>GSQGHDTVQPNFQQDKFLGRWY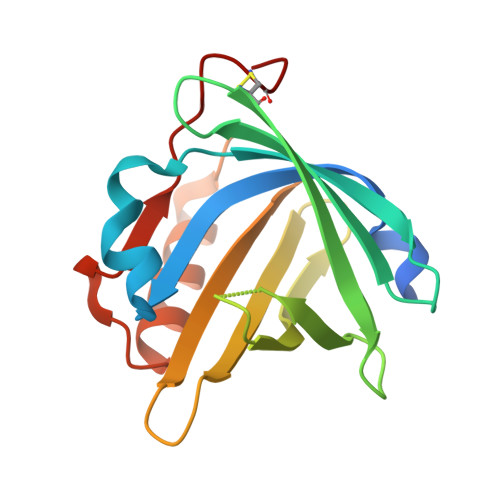SAGLASNSSWFREKKAVLYMAKTVVAPSTEGGLNLTSTFLRKNQCETKIMVLQPAGAPGHYTYSSPHSGSIHSVSVVEANYDEYALLFSRGTKGPGQDFRMATLYSRTQTLKDELKEKFTTFSKAQGLTEEDIVFLPQPDKCIQE[2x]Modulation of voltage-gated potassium (Kv) channels by auxiliary subunits is central to the physiological function of channels in the brain and heart. Native Kv4 tetrameric channels form macromolecular ternary complexes with two auxiliary β-subunits—intracellular Kv channel-interacting proteins (KChIPs) and transmembrane dipeptidyl peptidase-related proteins (DPPs)—to evoke rapidly activating and inactivating A-type currents, which prevent the backpropagation of action potentials. Here we report cryo-electron microscopy structures of the Kv4.2–DPP6S–KChIP1 dodecamer complex, the Kv4.2–KChIP1 and Kv4.2–DPP6S octamer complexes, and Kv4.2 alone. Thus, our data suggest that two distinct modes of modulation contribute in an additive manner to evoke A-type currents from the native Kv4 macromolecular complex.

To investigate how DPPs modulate the properties of Kv4, we solved the structures of the human Kv4.2–DPP6S binary and Kv4.2–DPP6S–KChIP1 ternary complexes. However, the focused refinement improved the resolutions of the transmembrane and intracellular regions to 3.4 Å and 3.9 Å for the Kv4.2–DPP6S and Kv4.2–DPP6S–KChIP1 complexes, respectively. The structures revealed that one DPP6S binds to one Kv4.2 in both complexes through their transmembrane domains, forming an octamer for Kv4.2–DPP6S and a dodecamer for Kv4.2–DPP6S–KChIP1. In the structures of the Kv4.2–DPP6S and Kv4.2–DPP6S–KChIP1 complexes, the DPP6S transmembrane helix hydrophobically interacts with the voltage-sensing domain of Kv4.2, specifically at the lower half of S1 and the upper half of S2. Structures of the Kv4.2–DPP6S and Kv4.2–DPP6S–KChIP1 complexes adopt the S4 up and S6 open conformation, like those of Kv4.2 alone and Kv4.2–KChIP1. Structural comparisons of Kv4.2–DPP6S and Kv4.2–DPP6S–KChIP1 as well as that of Kv4.2 alone and Kv4.2–KChIP1 further support the role of KChIP1 as a modulator of the Kv4.2 S6 helix by stabilizing the conformations of the Kv4.2 N and C termini as well as the intracellular S6 helix. KChIP1 and DPP6S do not directly interact with each other in the Kv4.2–KChIP1–DPP6S ternary complex. The structure of the Kv4.2–DPP6S–KChIP1 dodecameric complex supports the additive contribution of KChIPs and DPPs to the modulation of Kv4s in the ternary complex.

>AAGVAAWLPFARAAAIGWMPVASGPMPAPPRQERKRTQDALIVLNVSGTRFQTWQDTLERYPDTLLGSSERDFFYHPETQQYFFDRDPDIFRHILNFYRTGKLHYPRHECISAYDEELAFFGLIPEIIGDCCYEEYKDRRRENAERLQDDADTDTAGESALPTMTARQRVWRAFENPHTSTMALVFYYVTGFFIAVSVIANVVETVPCGSSPGHIKELPCGERYAVAFFCLDTACVMIFTVEYLLRLAAAPSRYRFVRSVMSIIDVVAILPYYIGLVMTDNEDVSGAFVTLRVFRVFRIFKFSRHSQGLRILGYTLKSCASELGFLLFSLTMAIIIFATVMFYAEKGSSASKFTSIPAAFWYTIVTMTTLGYGDMVPKTIAGKIFGSICSLSGVLVIALPVPVIVSNFSRIYHQNQRADKRRAQKKARLARIRAAKSGSANAYMQSKRSGLLSNQLQSSEDEQAFVSKSGSSFETQHHHLLHCLEKTTNHEFVD[4x];>[2x]PEGLEQLEAQTNFTKRELQVLYRGFKNECPSGVVNEDTFKQIYAQFFPHGDASTYAHYLFNAFDTTQTGSVKFEDFVTALSILLRGTVHEKLRWTFNLYDINKDGYINKEEMMDIVKAIYDMMGKYTYPVLKEDTPRQHVDVFFQKMDKNKDGIVTLDEFLESCQEDDNIMRSLQLFQNVM;>[2x]EGLEQLEAQTNFTKRELQVLYRGFKNECPSGVVNEDTFKQIYAQFFPHGDASTYAHYLFNAFDTTQTGSVKFEDFVTALSILLRGTVHEKLRWTFNLYDINKDGYINKEEMMDIVKAIYDMMGKYTYPVLKEDTPRQHVDVFFQKMDKNKDGIVTLDEFLESCQEDDNIMRSLQLFQNVM;>AAAAKGIAIALLVILVICSLIVTSVILLTPA[2x];>AKGIAIALLVILVICSLIVTSVILLTPA[2x]> EGDAAAGEKVSKKCLACHTFDQGGANKVGPNLFGVFENTAAHKDNYAYSESYTE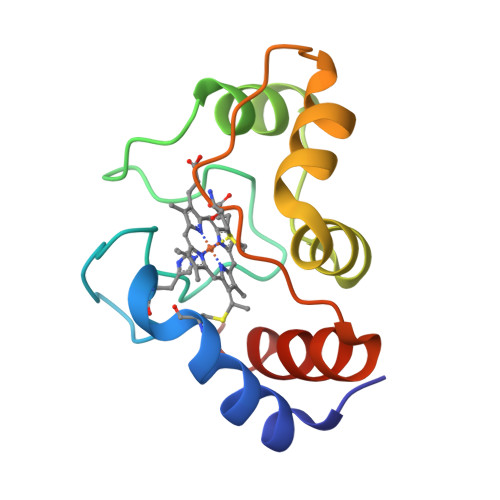MKAKGLTWTEANLAAYVKNPKAFVLEKSGDPKAKSKMTFKLTKDDEIENVIAYLKTLK> SNAMSYEEIAIQFASESVDATTIAAWVSEFAYQGFDARQVINLVKQRGGDDWKEDVKKMIVLSLTRGNKPSKMLNKMSESGQKIVNDL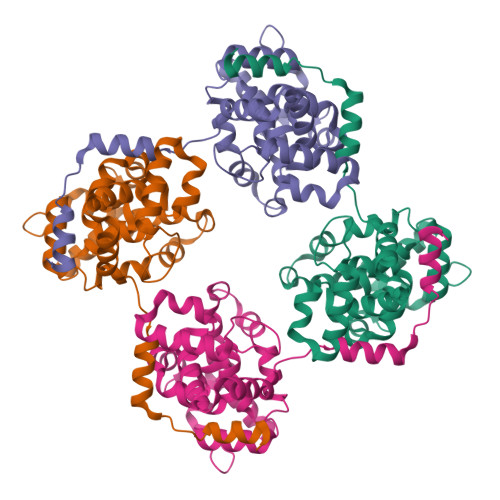ISKYKLKSGNPGRNDLTLSRIAAAFAGWTCQAAEVVQDYLPVTGRAMDAISDKFPRALMHPSFAGLVDPTLPEGVVEDIVHAHCLFMIQFSKTINPSLRSSSKSEVVSSFDRPMQAAINSPFLTAGNRRDILMSLGLINSNLKPSPTVVAAAKVYRKL>[4x]FQSITSPAKAVAKQENVVQLASEQPKVEMNKTAPSRFNGKERKVAYLTFDDGPGKYTAELLNTLKQHD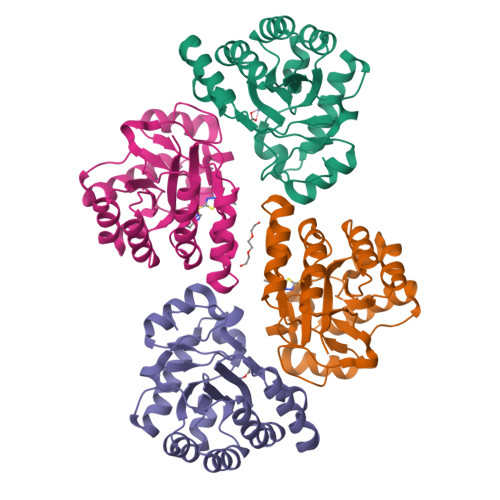AKATFFLIGANVKEFPDLVKRENAEGHYVGMHSMTHNFAKLYKNGEYVNEMKEDQGLIANIIGKSPKLTRPPYGSMPGLNEGLRNKVVEGGFKVWDWTIDSLDWRYNKMPVDAAAAQIAQNVLTNATKPQEVILMHDIHPQSVAAVPAILKGLKEKGYEFEAYHEESHFPVNFWHDNRM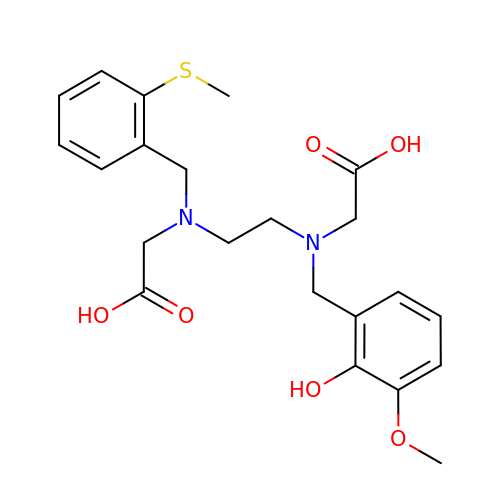2-[2-[2-hydroxy-2-oxoethyl-[(3-methoxy-2-oxidanyl-phenyl)methyl]amino]ethyl-[(2-methylsulfanylphenyl)methyl]amino]ethanoic acid | C22 H28 N2 O6 S | WFZIZUYYKZMMKQ-UHFFFAOYSA-N A prominent therapeutic target for antileishmanial drug development is leishmanial GDP-mannose pyrophosphorylase (GDP-MP or GMPP, EC 2.7.7.13), an enzyme catalyzing the formation of GDP-mannose by condensation of mannose-1-phosphate (Man-1-P) and GTP. As GDP-mannose serves as a central precursor for biosynthesis of diverse glycoconjugates necessary for host–parasite recognition and is essential for parasite survival, disruption of Leishmania GDP-MP activity leads to complete loss of virulence, suggesting this enzyme as an attractive target for development of new drugs against leishmaniasis. LdGDP-MP exhibits a hexameric structure with a molecular weight of ~245.3 kDa, consistent with previous observations. Each subunit is made of two separate domains, a N-terminal Rossmann-like fold commonly observed in nucleotidyltransferases and many other nucleotide-binding proteins, and a C-terminal left-handed β-helix domain containing tandem repeats of a [I/L/V]-G-X(4) hexapeptide motif, a characteristic structure found in the transferase hexapeptide repeat family.

We next solved the structure of LdGDP-MP in the absence of any cofactor or substrate at the resolution of 3.4 Å using single-particle cryo-EM imaging technique, which comprises of six subunits and exhibits a D3 symmetry with a dimension of ~104 Å × ~104 Å × ~108 Å. The homoheximeric LdGDP-MP complex is organized as a dimer of trimers, with each subunit pinched by two neighboring subunits via two interacting regions, namely, interface-1 and interface-2. In interface-1, the two subunits are attached in a shape-complementary manner between the region around the canonical signature motif GGXGXR(L)XPLX5PK of pyrophosphorylases (PPases)8 in one protomer and the C-terminus of another protomer; whereas interface-2 formation is mediated exclusively by the two C-terminal domains crossed at ~70 degrees. The contact surfaces for interface-1 and interface-2 amount to ~590 Å2 and ~750 Å2, respectively; and the interactions are established predominantly by hydrophobic interactions together with a few hydrogen bonds. Strikingly, replacement of R23 with alanine (R23A) caused loss of ~77% activity, whereas the mutations of P364N365 to arginines (PN), deletion of the last three residues on the C-terminus (ΔIIM), their combination (PN&ΔIIM), or deletion of the entire C-terminal domain (C-del) rendered the enzyme completely inactive, indicating the essential role of interprotomer communication in attaining leishmanial GDP-MP activity. On the other hand, disruption of the interface-1 contacts led to instability of the quaternary organization, as evidenced by drastic changes in the oligomerization status.

>[6x]MSASDGQGMRAVILVGGFGTRLRPLTLTTPKPLVPFCNKPMIIHQIEALKAVGVTEVILAVAYRPEAMKEQMDEWSRKLGVSFVFSVEEEPLGTAGPLALARDILMQDDKPFFVLNSDVTCTFPMQELLDFHKAHGGEGTIMVSQVTQWEKYGVVVYSPQNYQIERFVEKPSRFLGDRINAGIYIFNKSILDRIPPRRASIEKEIFPAMAAEGQLYAFNLEGFWMDVGQPKDYILGMTKFIPSLVHGNRETEQLHTEAVEHQRGGRFTVIGASLIDPSAKIGDGAVIGPYASIGANCVIGESCRIDNAAILENSKVGKGTMVSRSIVGWNNRIGSWCHIKDISVLGDDVEVKDGVILIGTKVLPNKDVGEHRFEPGIIM~{N}-[5-chloranyl-6-[(1~{S})-1-phenylethoxy]pyridin-3-yl]-2-(4-ethylsulfonylphenyl)ethanamide 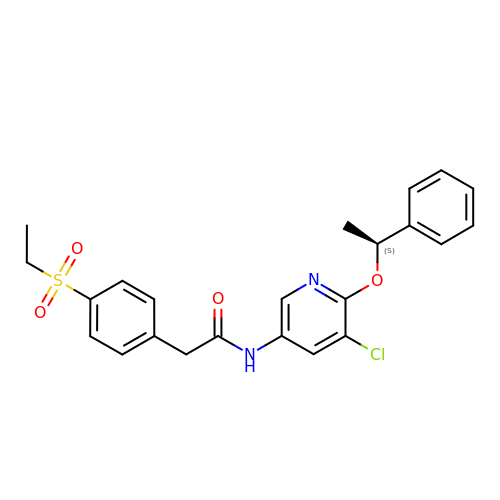| C23 H23 Cl N2 O4 S | VMHNMQCWPLURSW-INIZCTEOSA-N>MKKLFFALAMMLATVTAFLVAPSVKA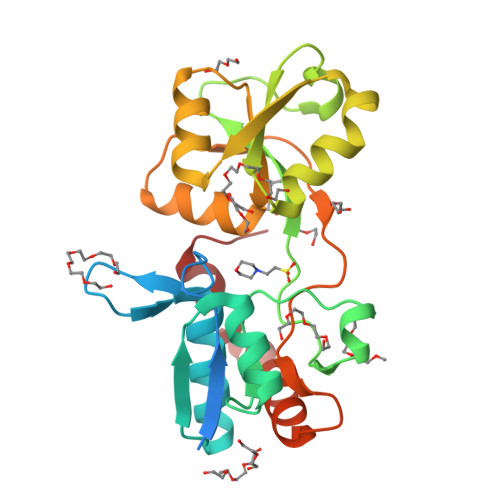ETTVKIASDSSYAPFEFQNGQKKWVGIDVDIMQEVAKINDWKLEMSYPGFDAALQNLKAGQVDGIIAGMTITDERKETFDFSNPYYTSALTIATTKDSKLSDYSDLKGKAVGAKNGTAAQTWLQENQKKYGYTIKTYSDGVHMFAALSSGNIAGAMDEVPVISYAMKQGQDLAMNFPSISLPGGYGFAVMKGKNSTLVDGFNKALAEMKSNGDYDKILKKYGITA[2x]>MGFLKGKKGLIVGVANNKSIAYGIAQSCFNQGATLAFTYLNESLEKRVRPIAQELNSPYVYELDVSKEEHFKSLYNSVKKDLGSLDFIVHSVAFAPKEALEGSLLETSKSAFNTAMEISVYSLIELTNTLKPLLNNGASVLTLSYLGSTKYMAHYNVMGLAKAALESAVRYLAVDLGKHHIRVNALSAGPIRTLASSGIADFRMILKWNEINAPLRKNVSLEEVGNAGMYLLSSLSSGVSGEVHFVDAGYHVMGMGAVEEK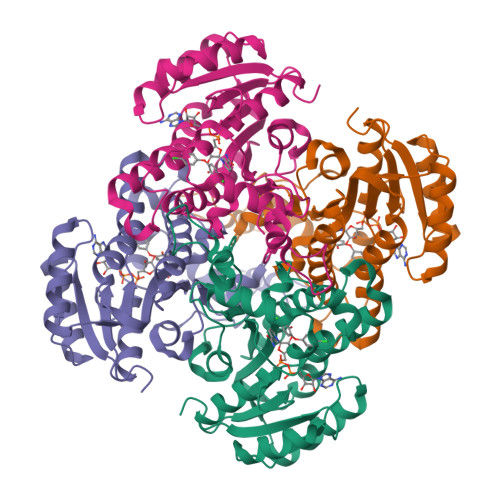DNKATLLWDLHKEQ[4x]>[4x]MLPSQSPAIFTVSRLNQTVRLLLEHEMGQVWISGEISNFTQPASGHWYFTLKDDTAQVRCAMFRNSNRRVTFRPQHGQQVLVRANITLYEPRGDYQIIVESMQPAGEGLLQQKYEQLKAKLQAEGLFDQQYKKPLPSPAHCVGVITSKTGAALHDILHVLKRRDPSLPVIIYPAAVQGDDAPGQIVRAIELANQRNECDVLIVGRGGGSLEDLWSFNDERVARAIFT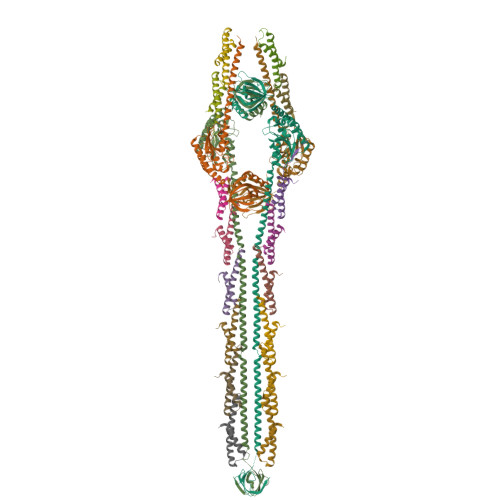SRIPVVSAVGAETDVTIADFVADLRAPTPSAAAEVVSRNQQELLRQVQSTRQRLEMAMDYYLANRTRRFTQIHHRLQQQHPQLRLARQQTMLERLQKRMSFALENQLKRTGQQQQRLTQRLNQQNPQPKIHRAQTRIQQLEYRLAETLRAQLSATRERFGNAVTHLEAVSPLSTLARGYSVTTATDGNVLKKVKQVKAGEMLTTRLEDGWIESEVKNIQPVKKSRKKVH;>MPKKNEAPASFEKALSELEQIVTRLESGDLPLEEALNEFERGVQLARQGQAKLQQAEQRVQILLSDNEDASLTPFTPDNE[16x]> MDVLSKGSLKELLAHLEKTPLEEAISYRIGTVPYQNVLISRNEYYNQLYPDTTSLIDGVSREGQRNVNGLIMSIISYVVSGSGHYIPNIGFMLLRRSILDILTKHDTGLVTNNLNYGIIARNLTVSKMNCEQRKRMLICFKLL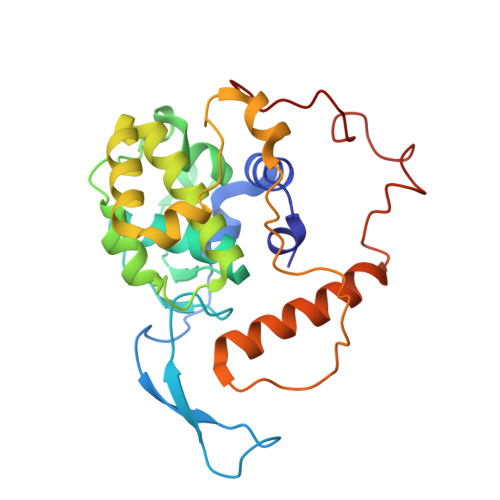AYKDGNQNDYEIYLNQNIPLKQIAPNFIPGDMRTVIHNQDQLAIVGIPAYRLTQSTELSIRDDNAKSYKLGYVDWYNSNSFLRERSEFNLIRLKDRDTKYGKLNGW> ESLVCNLRQLKCHFTWNLIAEDESLDEFEDRVFNKDEFQNSEFKATMCNILAYVKHCRGLNEAALQCLGEAEGFIQQQHPDQVEIRSLVTWGNYAWVYYHMGQFSKAQAYLDKVKQVCKKFSSPYRIENPALDCEEGWARLKCTKNQNERVKVCFQK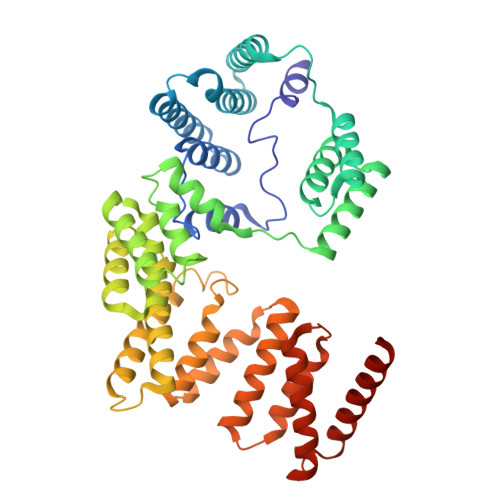ALEKDPKNPEFTSGWAIANYRLDDWPARNYCIDSLEQAIQLSPDNTYVKVLLALKLDAVHKNQAMALVEEALKKDPSAIDTLLRAARFYCKVYDTDRAIQLLRKALEKLPNNAYVHYYMGCCYRSKVHHMLNRREMVFSGDRKKLEELIQLAVNHLRKAEEIKEMLEYSCSFLADLYIIAKKYDEADYYFQKELSKDLPPGPKQLLHLRYGNFQFFQMKRQDKAIYHYMEGVKIKKKTIPQKKMREKLQRIALRRLHEDESDSEALHILAFLQENGGGQQADK> GSQGHDTVQPNFQQDKFLGRWYSAGLASNSSWFREKKAVLYMAKTVVAPSTEGGLNLTSTFLRKNQCETKIMVLQPAGAPGHYTYSSPHSGSIHSVSVVEANYDEY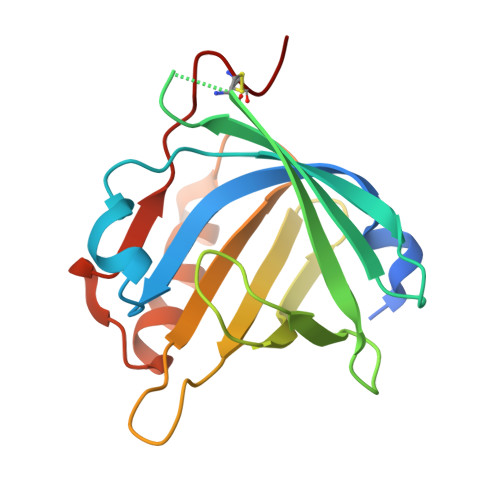ALLFSRGTKGPGQDFRMATLYSRTQTLKDELKEKFTTFSKAQGLTEEDIVFLPQPDKCIQE> MENTENSVDSKSIKNLEPKIIHGSESMDSGISLDNSYKMDYPEMGLCIIINNKN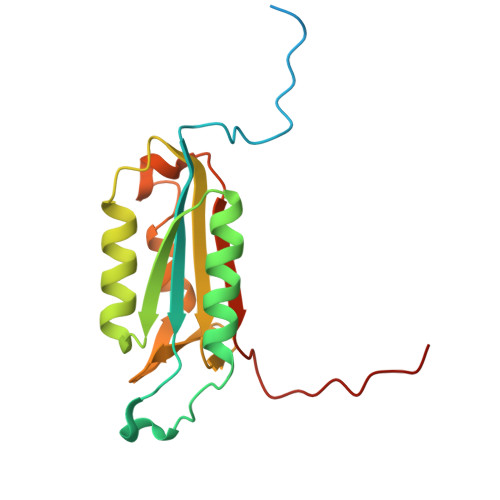FHKSTGMTSRSGTDVDAANLRETFRNLKYEVRNKNDLTREEIVELMRDVSKEDHSKRSSFVCVLLSHGEEGIIFGTNGPVDLKKITNFFRGDRCRSLTGKPKLFIIQACRGTELDCGIETD> AQSVPYGVSQIKAPALHSQGYTGSNVKVAVIDSGIDSSHPDLKVAGGASMVPSETNPFQDNNSHGTHVAGTVAALNNSIGVLGVAPSASLYAVKVLGADGSGQYSWIINGIEWAIANNMDVINMSLGGPSGSAALKAAVDKAVASGVVVVAAAGNEGTSGSSSTVGYPGKYPSVIAVGAVDSSNQRASFSSVGPELDVMAPGVSIQSTLPGNKYGAYNGTSMASPHVAGAAALILSKHPNWTNTQVRSSLENT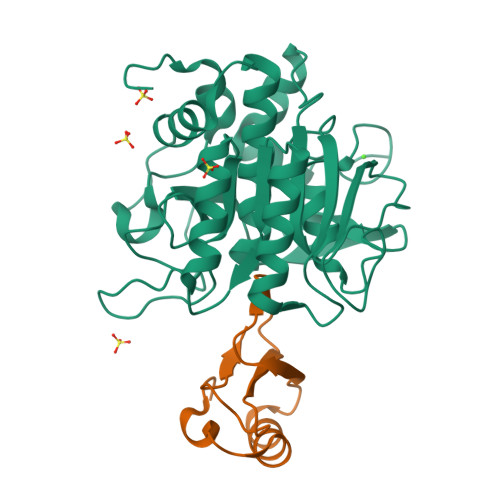TTKLGDSFYYGKGLINVQAAAQHHHHHH;> MKTEWPELVGKSVEEAKKVILQDKPAAQIIVLPVGTIVTMEYRIDRVRLFVDKLDNIAQVPRVG>[2x]GKSKAELQSEERKRIDELIESGKEEGMKIDLIDGKGRGVIATKQ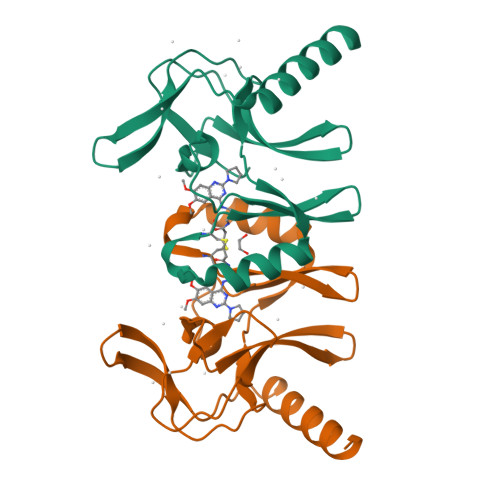FSRGDFVVEYHGDLIEITDAKKREALYAQDPSTGCYMYYFQYLSKTYCVDATRETNRLGRLINHSKSGNCQTKLHDIDGVPHLILIASRDIAAGEELLYDYGDR>PIYDLIIKNGIICTASDIYAAEIAVNNGKVQLIAASIDPSLGSEVIDAEGAFITPGGIDA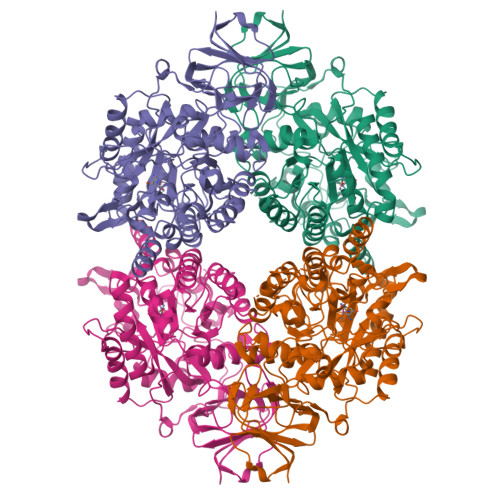HVHVDEPLKLLGDVVDTMEHATRSAVAGGTTTVVAFSTQDVSKKGPSALAESVKLDVDEYSEQTLYCDYGLHLILFQIEKPSVEARELLDVQLQAAYNDYGVSSVKMFMTYPGLQISDYDIMSAMYATRKNGFTTMLHAENGDMVKWMIEALEEQGLTDAYYHGVSRPSIVEGEATNRAITLATTMDTPILFVHVSSPQAAEVIKQAQTKGLKVYAETCPQYALLSDAITRCHHHGEVESYGVGIDLSSISESPFTNPDDRFIGSKYICSPPIRPEGTQKSIWKGMNNGTFTIVGSDHCSYNYYEKTSTASKHRAFDPENNKNGEFRYIPNGLPGVCTRMPLLYDYGYLRGNLTSMMKLVEIQCTNPAKVYGMYPQKGSILPGVSDADLVIWYPDDSKKEYNSKPKLITNKLMEHNCDYTPFEGIEIKNWPRYTIVKGKIVYKEGEILKENADGKYLKRGKSFMCTPKNEWVTEWRPKYESPGDDDDKHHHHHHHHSGD[4x]>HMRLELPVIPLRNTVILPHTTTPVDV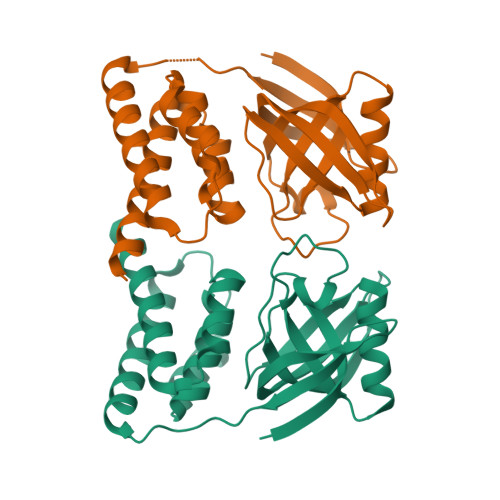GRAKSKRAVEEAMGADRLIFLVAQRDPEVDDPAPDDLYTWGVQAVVKQAMRLPDGTLQVMVEARARAQVTDYIPGPYLRARGEVFSEIFPIDEAVVRVLVEELKEAFEKYVANHKSLRLDRYQLEAVKGTSDPAMLADTIAYHATWTVAEKQEILELTDLEARLKKVLGLLSRDLERFELD[2x]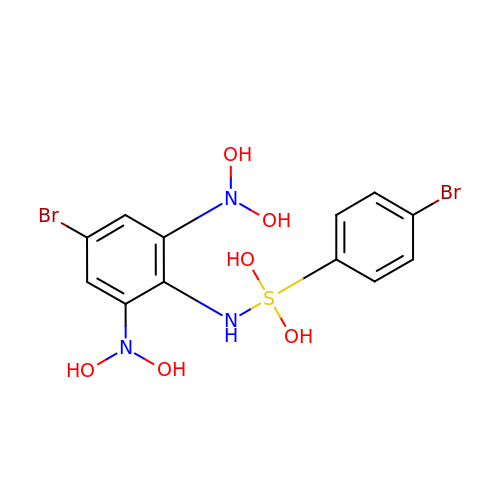5-bromanyl-N2-[(4-bromophenyl)-bis(oxidanyl)-$l^4-sulfanyl]-N1,N1,N3,N3-tetrakis(oxidanyl)benzene-1,2,3-triamine | C12 H13 Br2 N3 O6 S | NHTMTRVPPRZTCB-UHFFFAOYSA-N>[2x]GLSKEQESIIKLAENGHNIFYTGSAGTGKSILLREMIKVLKGIYGRENVAVTASTGLAACNIGGITIHSFAGIGLGKGDADKLYKKVRRSRKHLRRWENIGALVVDEISMLDAELLDKLDFIARKIRKNHQPFGGIQLIFCGDFFQLPPVSKDPNRPTKFAFESKAWKEGVKMTIMLQKVFRQRGDVKFIDMLNRMRLGNIDDETEREFKKLSRPLPDDEIIPAELYSTRMEVERANNSRLSKLPGQVHIFNAIDGGALEDEELKERLLQNFLAPKELHLKVGAQVMMVKNLDATLVNGSLGKVIEFMDPE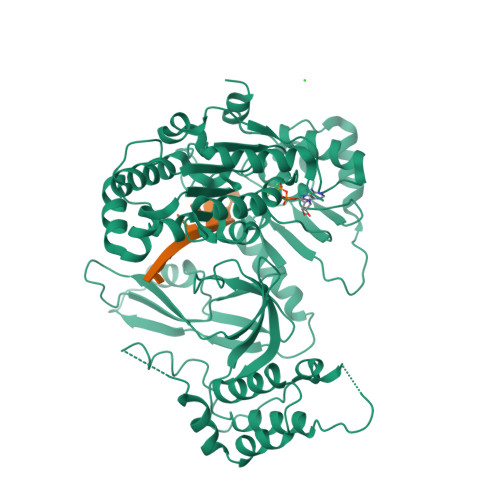TYFCYEALTNDPSMPPEKLETWAENPSKLKAAMEREQSDGEESAVASRKSSVKEGFAKSDIGEPVSPLDSSVFDFMKRVKTDDEVVLENIKRKEQLMQTIHQNSAGKRRLPLVRFKASDMSTRMVLVEPEDWAIEDENEKPLVSRVQLPLMLAWSLSIHKSQGQTLPKVKVDLRRVFEKGQAYVALSRAVSREGLQVLNFDRTRIKAHQKVIDFYLTLSSAESAYKQLEADEQV> GPGSASCLELALEGERLCKSGDCRAGVSFFEAAVQVGTEDLKTLSAIYSQLGNAYFYLHDYAKALEYHHHDLTLARTIGDQLGEAKASGNLGNTLKVLGNFDEAIVCCQRHLDISRELNDKVGEARALYNLGNVYHAKGKSFGCPGPQDTGEFPEDVRNALQAAVDLYEENLSLVTALGDRAAQGR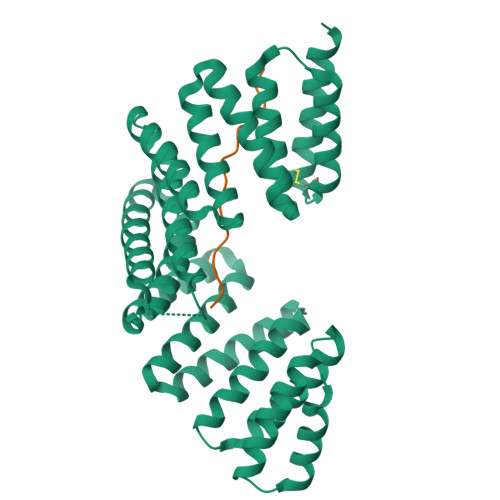AFGNLGNTHYLLGNFRDAVIAHEQRLLIAKEFGDKAAERRAYSNLGNAYIFLGEFETASEYYKKTLLLARQLKDRAVEAQSCYSLGNTYTLLQDYEKAIDYHLKHLAIAQELKDRIGEGRACWSLGNAYTALGNHDQAMHFAEKHLEISREVGD;> TNQHFVMVEVHRPDSEPDVNEVRALPQTRT>MAQLSGQPVVILPEGTQRYVGRDAQRLNILA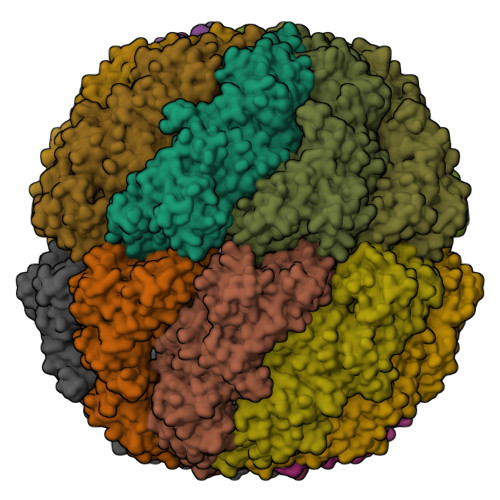ARIIAETVRTTLGPKGMDKMLVDSLGDIVVTNDCATILDKIDLQHPAAKMMVEVAKTQDKEAGDGTTTAVVIAGELLRKAEELLDQNIHPSIITKGYALAAEKAQEILDEIAIRVDPDDEETLLKIAATSITGKNAESHKELLAKLAVEAVKQVAEKKDGKYVVDLDNIKFEKKAGEGVEESELVRGVVIDKEVVHPRMPKRVENAKIALINEALEVKKTETDAKINITSPDQLMSFLEQEEKMLKDMVDHIAQTGANVVFVQKGIDDLAQHYLAKYGIMAVRRVKKSDMEKLAKATGAKIVTNVKDLTPEDLGYAEVVEERKLAGENMIFVEGCKNPKAVTILIRGGTEHVIDEVERALEDAVKVVKDVMEDGAVLPAGGAPEIELAIRLDEYAKQVGGKEALAIENFADALKIIPKTLAENAGLDTVEMLVKVISEHKNRGLGIGIDVFEGKPADMLEKGIIEPLRVKKQAIKSASEAAIMILRIDDVIAAKATKPEGGQGGGMPGGMGGMDMGM[4x]> GAMGEELTLTILRQTGGLGISIAGGKGSTPYKGDDEGIFISRVSEEGPAARAGVRV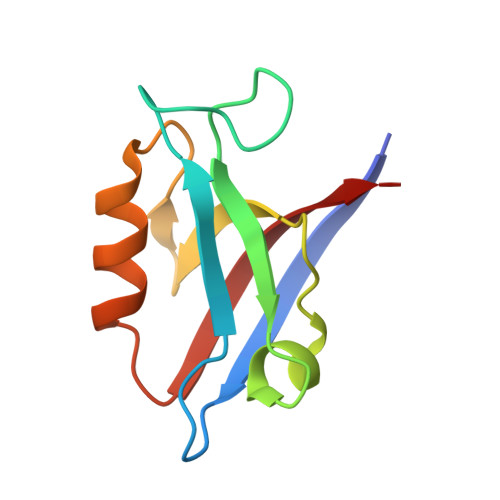GDKLLEVNGVALQGAEHHEAVEALRGAGTAVQMRVWRER7-[2-methoxy-6-[(4-methylpyridin-2-yl)methoxy]phenyl]-2,3,4,5-tetrahydro-1~{H}-3-benzazepine 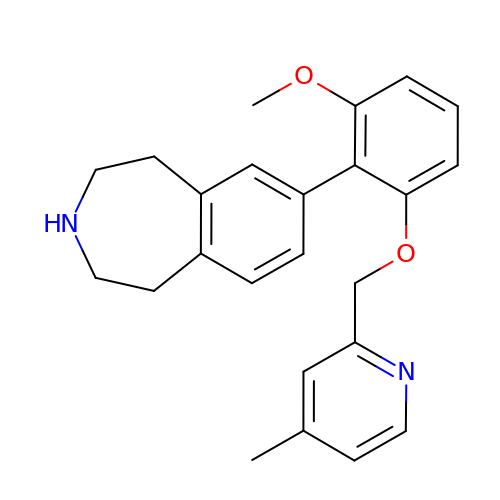| C24 H26 N2 O2 | KYANYGKXMNYFBX-UHFFFAOYSA-N> HTPVRTVMNTIQQLMMILNSASDQPSENLISYFNNCTVNPKESILKRVKDIGYIFKEKFAKAVGQGCVEIGSQRYKLGVRLYYRVMESMLKSEEERLSIQNFSKLLNDNIFHMSLLACALEVVMATYSRSTSQNLDSGTDLSFPWILNVLNLKAFDFYKVIESFIKAEGNLTREMIK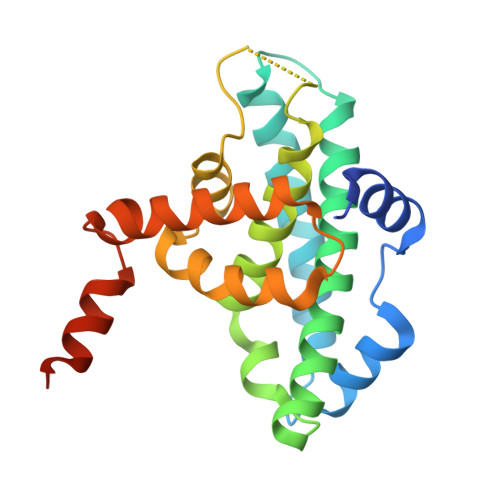HLERCEHRIMESLAWLSDSPLFDLIKQSKDREGPTDHLESA>[2x]MDKFRVQGPTRLQGEVTISGAKNAALPILFAALLAEEPVEIQNVPKLKDIDTTMKLLTQLGTKVERDGSVWIDASNVNNFSAPYDLVKTMRASIWALGPLVARFGQGQVSLPGGCAIGAAPVDLHIFGLEKLGAEIKLEEGYVKASVNGRLKGAHIVMDKVSVGATVTIMSAATLAEGTTIIENAAREPEIVDTANFLVALGAKISGQGTDRITIEGVERLGGGVYRVLPDRIETGTFLVAAAISGGK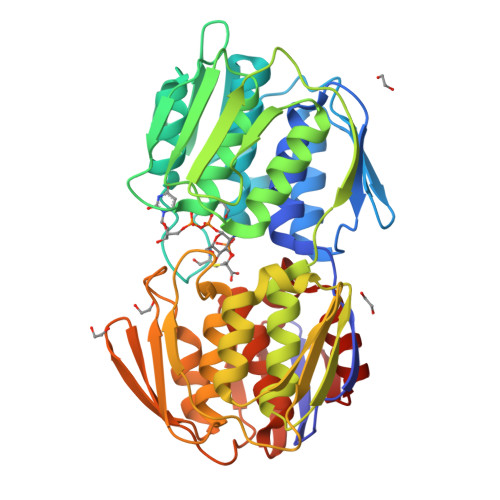IVCRNAQPDTLDAVLAKLREAGADIETGEDWISLDMHGKRPKAVTVRTAPHPAFPTDMQAQFTLLNLVAEGTGVITETIFENRFMHVPELIRMGAHAEIESNTVICHGVEKLSGAQVMATDLRASASLVLAGCIAEGTTVVDRIYHIDRGYERIEDKLRALGANIERVKGE Type IA topoisomerases (TopoIAs) are present in all living organisms. They resolve DNA/RNA catenanes, knots and supercoils by breaking and rejoining single-stranded DNA/RNA segments and allowing the passage of another nucleic acid segment through the break. Topoisomerase III-β (TOP3B), the only RNA topoisomerase in metazoans, promotes R-loop disassembly and translation of mRNAs. We present a series of cryo-EM structures of human TOP3B with its cofactor TDRD3 during cleavage and rejoining of DNA or RNA, thus elucidating the roles of divalent metal ions and key enzyme residues in each step of the catalytic cycle.

To study the structures of full-length TOP3B-TDRD3 in the presence and absence of DNA, we purified the human TOP3B(Y336F)-TDRD3 heterodimer from HEK293T cells. We first obtained an apo form TOP3B-TDRD3 map at ~3.1 Å resolution, which revealed the structure of TOP3B spanning amino acids 1–717, including half of its CTD (residues 612–717) as well as the N-terminal region of TDRD3 (residues 1–190). The planar assembly of the protein complex exhibits substantial positively charged surface areas on one side, which may enhance its binding to nucleic acids. Three Zn2+-binding motifs within the CTD of TOP3B were well defined, but the fourth and fifth C-4 zinc fingers (residues 718–815), as predicted by AlphaFold (AlphaFold DB O95985), are too mobile to be captured. Different from Zinc finger or zinc finger-like motifs in E. coliTOP1 and MtbTOP1, our structure reveals that TOP3B’s CTD establishes intramolecular contacts with both the core and an extended loop (residues 168–190) of TDRD3. The TOP3B-TDRD3 heterodimer is further stabilized by TOP3Bcore-TDRD3 contacts involving hydrophobic interactions of the extended loop of TDRD3 with two antiparallel TOP3B α-helices of domain IV.

> HMKTVLMVAEKPSLAQSIAKILSRGSLSSHKGLNGACSVHEYTGTFAGQPVRFKMTSVCGHVMTLDFLGKYNKWDKVDPAELFSQAPTEKKEANPKLNMVKFLQVEGRGCDYIVLWLDCDKEGENICFEVLDAVLPVMNKAHGGEKTVFRARFSSITDTDICNAMACLGEPDHNEALSVDARQELDLRIGCAFTRFQTKYFQGKYGDLDSSLISFGPCQTPTLGFCVERHDKIQSFKPETYWVLQAKVNTDKDRSLLLDWDRVRVFDREIAQMFLNMTKLEKEAQVEATSRKEKAKQRPLALNTVEMLRVASSSLGMGPQHAMQTAERLYTQGYISYPRTETTHYPENFDLKGSLRQQANHPYWADTVKRLLAEGINRPRKGHDAGDHPPITPMKSATEAELGGDAWRLYEYITRHFIATVSHDCKYLQSTISFRIGPELFTCSGKTVLSPGFTEVMPWQSVPLEESLPTCQRGDAFPVGEVKMLEKQTNPPDYLTEAELITLMEKHGIGTDASIPVHINNICQRNYVTVESGRRLKPTNLGIVLVHGYYKIDAELVLPTIRSAVEKQLNLIAQGKADYRQVLGHTLDVFKRKFHYFVDSIAGMDELMEVSFSPLAATGKPLSRCGKCHRFMKYIQAKPSRLHCSHCDETYTLPNNGTIKLYKELRCPLDDFELVLWSSGSRGKSYPLCPYCYNHPPFRDMKKGMGCNECTHPSCQHS;> MAQVAGAALSQAGWYLSDEGIEACTSSPDKVNVNDIILIALNTDLRTIGKKFLPSDINSGKVEKLEGPCVLQIQKIRNVAAPKDNEESQAAPRMLRLQMTDGHISCTAVEFSYMSKISLNTPPGTKVKLSGIVDIKNGFLLLNDSNTTVLGGEVEHLIEKWELQRSLSKHNRSNIGTEGGPPPFVPFGQ3-(4-piperidyl)propanoic acid | C8 H15 N O2 | 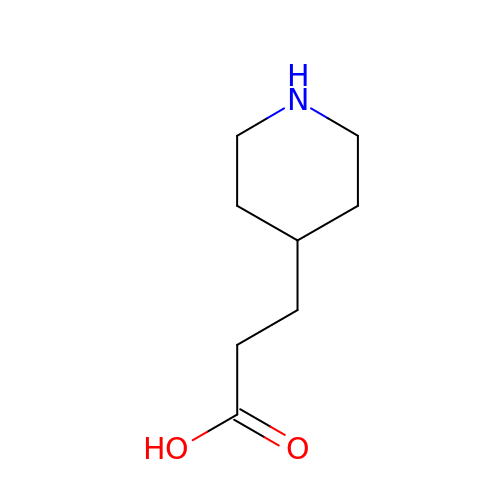AUYQMCCWFNSFGV-UHFFFAOYSA-N(2~{Z})-2-(1-oxidanyl-3-oxidanylidene-propyl)iminobutanedioic acid | C7 H9 N O6 | 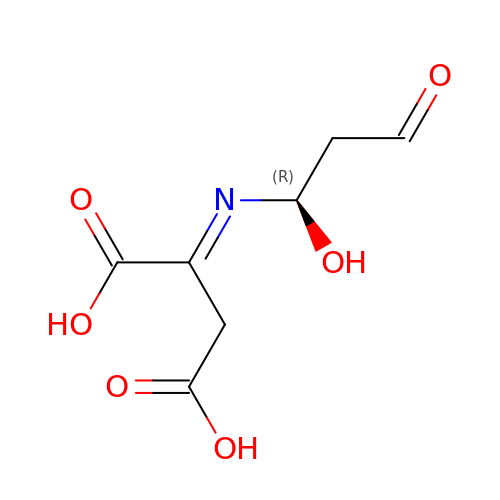BKMLHLNYNPUNII-RZTYMHDWSA-N> MSLSSWRQFQLFENIPIRDPNFGGDSLLYSDPTLCAATIVDPQTLIIAVNSNIIKVVKLNQSQVIHEFQSFPHDFQITFLKVINGEFLVALAESIGKPSLIRVYKLEKLPNREQLYHSQVELKNGNNTYPISVVSISNDLSCIVVGFINGKIILIRGDISRDRGSQQRIIYEDPSKEPITALFLNNDATACFAATTSRILLFNTTGRNRGRPSLVLNSKNGLDLNCGSFNPATNEFICCLSNFIEFFSSSGKKHQFAFDLSLRKRIFCVDKDHILIVTEETGVP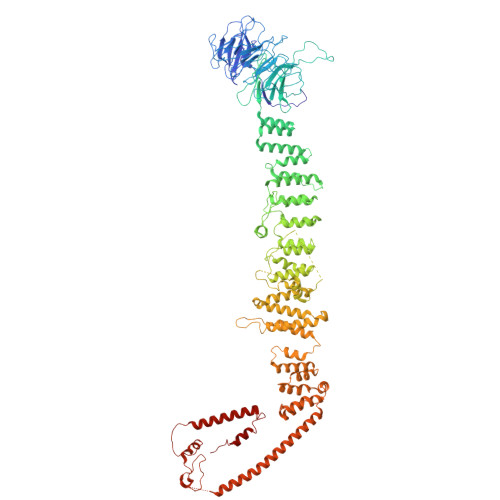TTSISVNELSPTIINRIFIIDAKNKIISLNFVVSSAIIDIFSTSQSGKNITYLLTSEGVMHRITPKSLENQINIIIQKELYPFALQLAKQHSLSPLDVQEIHKKYGDYLFKKGLRKEATDQYIQCLDVVETSEIISKFGVKEVPDPESMRNLADYLWSLIKNSISQRDHVTLLLIVLIKLKDVEGIDTFIQHFDRKGIWNEGVVMDDMDDVTFFYSDNDFFDLDLILELMKESDFKRLSYRLAKKYSKDSLIIVDILLNLLHNPVKAIKYIKSLPIDETLRCLVTYSKKLLEESPNETNALLIEVFTGKFKPSTFEVDLDRRDTTGDFSENIRTVFYSYKTFFNYMNSNGTSDAMSESSEASHEHEEPTYHPPKPSIVFSSFVTKPFEFVVFLEACLACYQQYEGFDEDRQVILTTLYDLYLNLAQNDVPERIDDWRSRATGVLRESNKLVYSAASNNTSKRVDNSIMLLISHMDQSSASAKDKTKIDIASFANDNPEMDLLSTFRAMTLNEEPSTCLKFLEKYGTEEPKLLQVALSYFVSNKLIFKEMGGNEVLKEKVLRPIIEGERMPLLDIIKALSRTNVAHFGLIQDIIIDHVKTEDTEIKRNEKLIESYDKELKEKNKKLKNTINSDQPLHVPLKNQTCFMCRLTLDIPVVFFKCGHIYHQHCLNEEEDTLESERKLFKCPKCLVDLETSNKLFEAQHEVVEKNDLLNFALNSEEGSRDRFKVITEFLGRGAISYSDITI> NTGLLESQLSRHDQMLSVHDIRLADMDLRFQVLETASYNGVLIWKIRDYKRRKQEAVMGKTLSLYSQPFYTGYFGYKMCARVYLNGDGMGKGTHLSLFFVIMRGEYDALLPWPFKQKVTLMLMDQGSSRRHLGDAFKPDPNSSSFKKPTGEMNIASGCPVFVAQTVLENGTYIKDDTIFIKVIVDTSDLPDPHHHHHH;> PSCPKPVQDTQPPES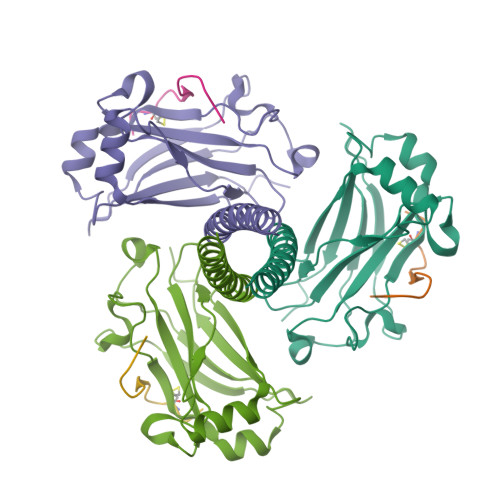PVENSE>MVIYGTGIDLTELSRIEAILAKGLRLPEKILTPAELAVFSRYPVKRQIEFMAGRFSAKEAYSKAYGTGIGAAVGFQDIEILDNAQGKPEVTRHPFDGPAWISISHTDTLVMTQVILERGNL[3x];>MTMDDTKATVLSILADLTGEDVSSNMDVNLFDEGILDSMGSVQLLLELQNQLGIEVPVSEFQRSEWDTPAKIVAKVENLQLEHHHHHH[3x]

TA d-alanylation is performed by the Dlt pathway, which starts in the cytoplasm and continues extracellularly after d-Ala transportation through the membrane. The first step in the d-alanylation mechanism of TA is the transfer of the phosphopantetheinyl moiety of coenzyme A (Ppant) to the DltC protein by the Phosphopantetheinyl transferase AcpS. The d-alanine-d-alanyl carrier protein ligase (DltA) catalyzes a two-step reaction: the activation of d-Ala using ATP to form a d-alanyl-AMP intermediate and then the transfer of d-Ala as a thiol ester to the Ppant group of DltC. Altogether, we conclude that DltC1 acts as an interaction hub for all the successive cytoplasmic steps of the TA d-alanylation pathway.

High quality diffracting crystals were obtained and the crystal structure was solved at 1.88 Å resolution. We first confirmed the trimeric assembly of the AcpS-DltC1 complex and brought new evidence that two AcpS monomers are required to dock one DltC1 molecule during the catalytic reaction. The interface between two adjacent AcpS monomers serves as a docking area for DltC1 binding. The first one is the largest and locates at the interface between the helix α2 and the loop connecting helices α2 and α3 of DltC1 and the helix α1 of one adjacent AcpS monomer. One is strictly conserved in B. subtilis and is established between the well conserved Arg15 of AcpS and Asp37 of DltC1, the latter being located just before the reactive Serine. The Asp32 of DltC1 located in the long loop between helices α1 and α2 forms a strong ionic interaction with Arg46 of AcpS and an H-bond with Tyr42. A clear electron density, corresponding to a phosphate moiety of Ppant, was observed covalently linked to the Ser38 side chain in only one of the 3 subunits of DltC1 of the complex. Indeed, although covalently linked to Ser38, it points toward a neighboring AcpS molecule and ends in the vicinity of the end of β2 and the beginning of α4. In this position, the thiol group at the extremity of the Ppant is stabilized via H-bond interactions with Glu49, Asp82 and the well conserved Arg46 of AcpS. Our finding that the AcpS/DltC1 cannot form a complex when DltC1 is fully Ppanted provides the molecular basis for the dissociation of the AcpS-DltC1 complex allowing subsequent DltC1 binding to DltA.> MSSSFVSNGASLEDCHCNLFCLADLTGIKWKRYVWQGPTSAPILFPVTEEDPILSSFSRCLKADVLGVWRRDQRPGRRELWIFWWGKDPNFADLIHHDLSEEEDGVWENGLSYECRTLLFKAVHNLLERCLMNRNFVRIGKWFVKPYEKDEKPINKSEHLSCSFTFFLHGDSNVCTSVEINQHQPVYLLSEEHVTLAQQSNSPFQVILSPFGLNGTLTGQAFKMSDSATKKLIGEWKQFYPISCGLKEMSEEKQDDMDWEDDSLAAVEVLVAGVRMIYPACFVLVPQSDIPAPSSVGASHCSASCLGIHQVPASTRDPAMSSVTLTPPTSPEEVQTVDPQSAQKWVKFSSVSDGFSTDSTSHHGGKIPRKLANHVVDRVWQECNMNRLQNKRKYSATSSGLCEEETADKIGCWDFVEATQRTSCSCLRHKSLKTRNTGQQGQAPSLGQQQQVLPKHKTNEKQDKSEKPQKRPLTPFHHRVSVSDEIGMDTDSASQRLVISAADSQVRFSNIRTNDVAKTPQMHGTELANSPQPPPLSPHPCDVVDEGVTKTPSTPQSQHFYQMPTPDPLVPTKPMEDRIDSLSQSFPPPFQEAVEPTVYVGTAVSLEEDEANVAWKYYKVPKKKDVEFLPPQLPNDKFKDDPVGPFGQESVTSVTELMVQCKKPLKVSDEIVQQYQIKNQYLSAIASDTEQEPKIDPYAFVEGDEEFIFTDKKDRQNSEREAGKKHKVEDGTSAVTVLSHEEDAMSLFSPSKQDAPRPTNHARPPSTSLIYDSDLAVSYTDLDNLFNSDEDELTPGSKKSASGSDDKASSKESKTGNLDPLSCISTADLHKMYPTPPSLEQHIMGFSPMNMNNKEYGSVDTAPGGTVLEGNSSSVGTQFRIEVEEGFCSPKPSEIKDFSYVYKPENCQVLVGCSMFAPLKTLPSHCLPPIKLPEECVYRQSWTVGKLDLLPSGPSMPFIKEGDGSNLDQDYGPAYTPQTHASFGMPPSSAPPSNGGAGILPSPSTPRFPTPRTPRTPRTPRGAGGPASAQGSVKYENSDLYSPASTPSTCRPLNSVEPATVPSIPEAHSLYVNLILSESVMNLFKDCNFDSCCICVCNMNIKGADVGVYIPDPTQEAQYRCTCGFSAVMNRKFGNNSGLFLEDELDIIGRNTDCGKEAEKRFEALRASSVENVNGGLKESEKVPDELILLLQDQCTNLFSPFGAADQDPFPKVGISSNWVRVEERDCCSDCCLALEHGRQFMDNMSGGKVDEALVRSSCLHPWAKQNDASVQCSQDILRMLLSLQPVLQDAIQKKRTVRPWGVQGPLTWQQFHKMAGRGSYGTDESPEPLPIPTFLLGYDYDFLVLSPFALPYWEKLMLEPYGSQRDIAYVVLCPENEALLNGARSFFRDLTAIYESCRLGQHRPISRLLTDGIMKVGATASKKLSEKFVTEWFSQAADGNNEAFSKLKLYAQVCRYDLGPYLASQPLDSSLLSQPNLVAPPNQSLVTAPQMTNTGNANAPSATLASAASSTMTMTSGVPISTSVATANSTLTTTSSSSSSSLSSGVSSNKLPSFPPFGSMNTSGTGSMSAQASTVQSGQLGGQQSSSLQAAGISGESASLPTQPHPDVSESTMDRDKVGIPTDGDSHAITYPPAIVVYIIDPFTYENKDESTNSSNVWTLGLLRCFLEMVQTLPPHIKSTVSVQIVPCQYLLQPVKHDDRQIYSQHLKSLAFSVFTQCRRPLPTSTNVKTLTGFGPGLAMETALKSPDRPECIRLYTPPFILAPVKDKQTELGETFGEAGQKYNVLFVGYCLSHDQRWILASCTDLYGELLETCIINIDVPNRARRKKGSARRFGLQKLWEWCLGLVQMSSLPWRVVIGRLGRIGHGELKDWSCLLSRRNLQSLSKRLKDMCRMCGISAADSPSILSACLVAMEPQGSFVIMPDSVSTGSVFGRSTTLNMQTPQLNTPQDTSCTHILVFPTSASVQVASATYTTENLDLAFNPNNDGADGMGIFDLLDTGDDLDPDIINILPASPTASPVHSPGSHYPHGGDAGKGQGTDRLLSTESHDEVTNILQQPLALGYFVSTAKAGPLPDWFWSACPQAQYQCPLFLKASLHLHVPSVQSDELLHSKHSHPLDSNQTSDVLRFVLEQYNALSWLTCDPAVQDRRSCLPVHFVVLNQLYNFIMNML;> MKAQGETEDSERLSKMSSLLERLHAKFNQNRPWSETIKLVRQVMEKRVVMSSGGHQHLVSCLETLQKALKVTSLPAMTDRLESIARQNGLGSHLSASGTECYITSDMFYVEVQLDPAGQLCDVKVAHHGENPVSCPELVQQLREKNFEEFSKHLKGLVNLYNLPGDNKLKTKMYLALQSLEQDLSKMAIMYWKATNAAPLDKILHGSVGYLTPRSGGHLMNMKYYASPSDLLDDKTASPIILHEKNVPRSLGMNASVTIEGTSAMYKLPIAPLIMGSHPADNKWTPSFSAVTSANSVDLPACFFLKFPQPIPVSKAFVQKLQNCTGIPLFETPPTYLPLYELITQFELSKDPDPLPLNHNMRFYAALPGQQHCYFLNKDAPLPDGQSLQGTLVSKITFQHPGRVPLILNMIRHQVAYNTLIGSCVKRTILKEDSPGLLQFEVCPLSESRFSVSFQHPVNDSLVCVVMDVQDSTHVSCKLYKGLSDALICTDDFIAKVVQRCMSIPVTMRAIRRKAETIQADTPALSLIAETVEDMVKKNLPPASSPGYGMTTGNNPMSGTTTPTNTFPGGPITTLFNMSMSIKDRHESVGHGEDFSKVSQNPILTSLLQITGNGGSTIGSSPTPPHHTPPPVSSMAGNTKNHPMLMNLLKDNPAQDFSTLYGSSPLERQNSSSGSPRMEMCSGSNKAKKKKSSRVPPDKPKHQTEDDFQRELFSMDVDSQNPMFDVSMTADALDTPHITPAPSQCSTPPATYPQPVSHPQPSIQRMVRLSSSDSIGPDVTDILSDIAEEASKLPSTSDDCPPIGTPVRDSSSSGHSQSALFDSDVFQTNNNENPYTDPADLIADAAGSPNSDSPTNHFFPDGVDFNPDLLNSQSQSGFGEEYFDESSQSGDNDDFKGFASQALNTLGMPMLGGDNGEPKFKGSSQADTVDFSIISVAGKALGAADLMEHHSGSQSPLLTTGELGKEKTQKRVKEGNGTGASSGSGPGSDSKPGKRSRTPSNDGKSKDKPPKRKKADTEGKSPSHSSSNRPFTPPTSTGGSKSPGSSGRSQTPPGVATPPIPKITIQIPKGTVMVGKPSSHSQYTSSGSVSSSGSKSHHSHSSSSSSLASASTSGKVKSSKSEGSSSSKLSGSMYASQGSSGSSQSKNSSQTGGKPGSSPITKHGLSSGSSSTKMKPQGKPSSLMNPSISKPNISPSHSRPPGGSDKLASPMKPVPGTPPSSKAKSPISSGSSGSHVSGTSSSSGMKSSSGSASSGSVSQKTPPASNSCTPSSSSFSSSGSSMSSSQNQHGSSKGKSPSRNKKPSLTAVIDKLKHGVVTSGPGGEDPIDSQMGASTNSSNHPMSSKHNTSGGEFQSKREKSDKDKSKVSASGGSVDSSKKTSESKNVGSTGVAKIIISKHDGGSPSIKAKVTLQKPGESGGDGLRPQIASSKNYGSPLISGSTPKHERGSPSHSKSPAYTPQNVDSESESGSSIAERSYQNSPSSEDGIRPLPEYSTEKHKKHKKEKKKVRDKDRDKKKSHSMKPENWSKSPISSDPTASVTNNPILSADRPSRLSPDFMIGEEDDDLMDVALIGN;> MAASSSGEKEKERMGGVSGMAGLGSTRERLLSALEDLEVLSRELIEMLAISRNQKLLQLEEENQVLELLIHRDGDFQELMKLALNQGKVHHEMQALEKEVEKRDSDIQQLQKQLKEAEQILATAVYQAKEKLKSIEKARKGAISSEEIIKYAHRISASNAVCAPLTWVPGDPRRPYPTDLEMRSGLLGQMNNPSTSGVNGHLPGDALAAGRLPDVLAPQYPWQSNDMSVNMLPPNHSSDFLLEPPGHNKENEDDVEVMSTDSSSSSSDSD;> MAAVDIRDNLLGISWVDSSWIPILNSGSVLDYFSERSNPFYDRTCNNEVVKMQRLTLEHLNQMVGIEYILLHAQEPILFIIRKQQRQSPAQVIPLADYYIIAGVIYQAPDLGSVINSRVLTAVHGIQSAFDEAMSYCRYHPSKGYWWHFKDHEEQEKVKPKAKRKEEPSSIFQRQRVDALLIDLRQKFPPRFVQQKSGEKPVPVDQAKKEAEPLPETVKSEEKESTKNIQQTVSTKGPPEKRMRLQ;> MGEPQQVSALPPPPMQYIKEYTDENIQEGLAPKPPPPIKDSYMMFGNQFQCDDLIIRPLESQGIERLHPMQFDHKKELRKLNMSILINFLDLLDILIRSPGSIKREEKLEDLKLLFVHVHHLINEYRPHQARETLRVMMEVQKRQRLETAERFQKHLERVIEMIQNCLASLPDDLPHSEAGMRVKAEPMDTDDNSNCPGQNEQQRESSGHRRDQIIEKDAALCVLIDEMNERP;> MQREEKQLEASLDALLNQVADLKNSLGSFIYKLENEYDRLTWPSVLDSFALLSGQLNTLNKVLKHEKTPLFRNQVIIPLVLSPDRDEDLMRQTEGRVPVFSHEVVPDHLRTKPDPEVEEQEKQLTTDAARIGADAAQKQIQSLNKMCSNLLEKISKEERESESGGLRPNKQTFNPGDTNALVAAVAFGKGLSNWRPSGSSGPGQPGQPGAGTILAGASGLPQVQMPGAPNQQQPMLSGVQMAQAGQPGKMPSGIKTNIKSASMHPYQR;> MASSGVAGGRQAEDTLQPPPELLPESKPPPPPQPLPVAALPPPAAPRPQSPAGAKEENYSFLPLVHNVIKCMDKDSPDLHQDLNALKTKFQELRKLIGTMPGIHVSPEQQQQQLHSLREQVRTKNELLQKYKSLCMFEIPKD;> MAEKFDHLEEHLEKFVENIRQLGIIVSDFQPSSQAGLSQKLNFIVTGLQDIDKCRQQLHDITVPLEVFEYIDQGRNPQLYTKECLERALAKNEQVKGKIDTMKKFKSLLIQELSKVFPEDMAKYRSIRGEDHPPS;> MATYSLANERLRALEDIEREIGAILQNAGTAILELSKEKTNERLLDRQAAAFTTSVQHVEAELSAQIRYLTQVATGQPHEGSSYSSRKDCQMALKRVDYARLKISDVARTCEQMLEN;> MAPVQLDNHQLIPPGGGGGSSGGGGSSSGSASAPAPPPPAAAVAAAAAAAASPGYRLSTLIEFLLHRAYSELMVLTDLLPRKSDVERKIEIVQFASRTRQLFVRLLALVKWANDAGKVEKCAMISSFLDQQAILFVDTADRLASLARDALVHARLPSFAIPYAIDVLTTGSYPRLPTCIRDKIIPPDPITKIEKQATLHQLNQILRHRLVTTDLPPQLANLTVANGRVKFRVEGEFEATLTVMGDDPEVPWRLLKLEILVEDKETGDGRALVHSMQIDFIHQLVQSRLFADEKPLQDMYNCLHCFCLSLQLEVLHSQTLMLIRERWGDLVQVERYHAGKSLSLSVWNQQVLGRKTGTASVHKVTIKIDENDVSKPLQIFHDPPLPASDSKLVERAMKIDHLSIEKLLIDSVHARAHQRLQELKAILRSFNANESSSIETALPALIVPILEPCGNSECLHIFVDLHSGMFQLMLYGLDPATLEDMEKSLNDDMKRIIPWIQQLKFWLGQQRCKQSIKHLPTITTETLQLANYSTHPIGSLSKNKLFIKLTRLPQYYIVVEMLEVPNKPTQLSYNYYFMSVSTADREDSPVMALLLQQFKDNIQDLMSYTKTGKQTRTGTKHKLSDDPCPIDSKKAKRSGEMCAFNKVLAHFVAMCDTNMPFVGLRLELSNLEIPHQGVQVEGDGFNHAIRLLKIPPCKGISEETQKALDRSLLDCTFRLQGRNNRTWVAELVFANCPLNGTSTREQGPSRHVYLTYENLLSEPVGGRKVVEMFLNDWSSIARLYECVLEFARSLPEIPAHLNIFSEVRVYNYRKLILCYGTTKGSSISIQWNSIHQKFHIALGTVGPNSGCSNCHNTILHQLQEMFNKTPNVVQLLQVLFDTQAPLNAINKLPTVPMLGLTQRTNTAYQCFSILPQSSTHIRLAFRNMYCIDIYCRSRGVVAIRDGAYSLFDNSKLVEGFYPAPGLKTFLNMFVDSNQDARRRSVNEDDNPPSPIGGDMMDSLISQLQPPQQQPFPKQPGTSGAYPLTSPPTSYHSTVNQSPSMMHTQSPGNLHAASSPSGALRAPSPASFVPTPPPSSHGISIGPGASFASPHGTLDPSSPYTMVSPSGRAGNWPGSPQVSGPSPATRLPGMSPANPSLHSPVPDVSHSPRAGTSSQTMPTNMPPPRKLPQRSWAASIPTILTHSALNILLLPSPTPGLVPGLAGSYLCSPLERFLGSVIMRRHLQRIIQQETLQLINSNEPGVIMFKTDALKCRVALSPKTNQTLQLKVTPENAGQWKPDELQVLEKFFETRVAGPPFKANTLIAFTKLLGAPTHILRDCVHIMKLELFPDQATQLKWNVQFCLTIPPSAPPIAPPGTPAVVLKSKMLFFLQLTQKTSVPPQEPVSIIVPIIYDMASGTTQQADIPRQQNSSVAAPMMVSNILKRFAEMNPPRQGECTIFAAVRDLMANLTLPPGGRP;> MDVSGQETDWRSAAFRQKLVSQIEDAMRKAGVAHSKSSKDMESHVFLKAKTRDEYLSLVARLIIHFRDIHNKKSQASVSDPMNALQSLTGGPTPGAAGIGMPPRGPGQSLGGMGGLGAMGQPLPLSGQPPPGTSGMAPHGMAVVSTATPQTQLQLQQVALQQQQQQQQQQQFQQQQAALQQQQQQQQQQQQQQQFQAQQNAMQQQFQAVVQQQQLQQQQQQQHLIKLHHQSQQQQIQQQQLQRMAQLQLQQQQQQQQQQALQAQPPMQQPSMQQPQPPPSQALPQQLSQLHHPQHHQPPPQAQQSPIAQNQPPQIPPQSQSQPLVSQAQALPGPMLYAAQQQLKFVRAPMVVQQPQVQPQVQQVQPQVQPQAAVQAAQSAQMVAPGVQMIAEALAQGGMHVRARFPPTSTMSAGPSSSISLGGQPTTQVSQSSLTMLSSPSPGQQVQTPQSMPPPPQPSPQPGSQPNSNVSSGPAPSPSSFLPSPSPQPSQSPVTARTPQNFSVPSPGPLNTPVNPSSVMSPAGSSQAEEQQYLDKLKQLSKYIEPLRRMINKIDKNEDRKKDLSKMKSLLDILTDPSKRCPLKTLQKCEIALEKLKNDMAVPTPPPPPVLPTKQQDLCQPLLDAVLANIRSPVFNHSLYRTFVPAMMAIHGPPIVSPVVCSRKRRFEEDERQSIPNVLQGEVARLDPKFLVNLDPSHCSNNGTVHLICKLDDKDLPSVPPLELSVPADYPAQSPMWIDRQWQYDANPFLQSVHRCMTSRLLQLPDKHSVTALLNTWAQSIHQACLSAA;> MDLAYVCEWEKWAKSTYCPSLPLACAWSCRNLIAFTTDLRNDDQDLTHMIHILDTEHPWEVHSVSSGHSEAITCLEWDQSGSRLLSADADGQIKCWSMADHLANSWESSVGSQVEGDPIVALSWLHNGVKLALHVEKSGASSFGEKFSRVKFSPSLTLFGGKPMEGWIAVTVSGLVTVSLLKPSGQVLTSTESLCRLRGRVALADIAFTGGGNIVVAAADGSSASPVKFYKVCVSVVSEKCRIDTEILPSLFMRCTTDPNRKDRFPAITHLKFLARDMSEQVLLCASSQTSSLVECWSLRKEGLPVNNIFQQISPVVGDKQPMILKWRILSATNDLDRVSAVALPKLPISLTNTDLKVASDTQFYPGLGLALAFQDGSVHMVHRLSLQTMAVFYSSAPRSLDEPALKRPRTTCPAVHFKAMQLSWTSLALVGIDNHGKLSMLRISPSLGHPLEPKLALQHLLFLLEYCMVTGYDWWDILLHVQPGMVQSLVERLHEEYTRQKPALQQVLSTRILAMKASLCKLSPCTVARVCDYHTKLFLMAITSTLKSLLRPHFLNTPDKSPGDRLAEICAKITDVDIDKVMINLKTEEFVLDMNTLQALQQLLQWVGDFVLYLLVSLPNQGSPLRPGHSFLRDGTSLGMLRELMVVIRIWGLLKPSCLPVYTATSDTQDSMSLLFRLLTKLWICCRDEGAASEPDEGLVDECCLLPSQLLVPNLDWLPASDGLVSRLQPKQPLRLRFGRAPTLPSSTSTLQLDGLTRAPGQPKIDHLRRLHLGAYPTEECKACTRCGCVTMLKSPNKTTAVTQWEQRWIKNCLCGGLWRRVPLSCS;> MSGVRAVRISIESACEKQVQEVGLDGTETYLQPLSMSQNLARLAQRIDFSQGSGSEEEEAAGPDGDAPDWGGAGADQDDEEGLVKFQPSLWPWDSVRNNLRSALTEMCVLYDVLSIVRDKKFMTLDPVSQDALPPKQSPQTLQLISKKKSLAGAAQILLKGAERLTKSVAENQENKLQRDFNSELLRLRQHWKLRKVGDKILGDLSYRSAGSLFPHHGTFEVIKNTDIDLDKKIPEDYCPLDVQIPSDLEGSAYIKVSIQKQAPDIGDLGTVNLFKRPLPKSKPGSPHWQTKLEAAQNVLLCKEIFAQLSREAVQIKSQIPHIVVKNQIISQPFPSLQLSISLCHSSDDKKSQKCAAEKPGQEDHLYVLEHNLHLLIREFHKQTLSSIVMPHPASAPFGHKRMRLSGPQAFDKNEINSIQSTEGLLEKIIKQAKHIFLRSRTAATIDSLASRIEDPQIQAHWSNINDVYESSVKVLITSQGYEQICKSIQLQLNIGVEQVRVVHRDGRVIMLSHQEQELQDFLLSQMSQHQVHAVQQLAKVMGWQVLSFSNHVGLGPIESIGNASAITVASPSGDYAISVRNGPESGSKIMVQFPRNQCKDLPKSDVLQDSKWSHLRGPFKEVQWNKMEGRNFVYKMELLMSALSPCLL;> MEAPPVTMMPVTGGTINMMEYLLQGSVLDHSLESLIHRLRGLCDNMEPETFLDHEMVFLLKGQQASPFVLRARRSMDRAGAPWHLRYLGQPEMGDKNRHALVRNCVDIATSENLTDFLMEMGFRMDHEFVAKGHLFRKGIMKVVVYKIFRILVPGNTDSTEALSLSYLVELSVVAPAGQDMVSDDMRNFAEQLKPLVHLEKIDPKRLM;> MGVTCVSQMPVAEGKSLQQTVELLTKKLEMLGAEKQGTFCVDCETYHTAASTLGSQGQAGKLMYVMHNSEYPLSCFALFENGPCLIADTNFDVLMVKLKGFFQSAKASKIETRGTRYQYCDFLVKVGTVTMGPSARGISVEVEYGPCVVASDCWSLLLEFLQSFLGSHAPGAPTVFGNRHDAVYGPADTMIQYMELFNKIRKQQQVPVAGIR;> MADRLTQLQDAVNSLADQFCNAIGVLQQCGPPASFSNIQTAINKDQPANPTEEYAQLFAALIARTAKDIDVLIDSLPSEESTAALQAASLYKLEEENHEAATCLEDVVYRGDMLLEKIQSALADIAQSQLKTRSVTHSHSLPDS;> MAQQRALPQSKETLLQSYNKRLKDDIKSIMDNFTEIIKTAKIEDETQVSRATQGEQDNYEMHVRAANIVRAGESLMKLVSDLKQFLILNDFPSVNEAIDQRNQQLRALQEECDRKLITLRDEVSIDLYELEEEYYSSSSSLCEANDLPLCEAYWRLDLDADSADGLSAPLLASPETGAGPLQSAAPVHSHGGGPGPTEHT;> METQLQSIFEEVVKTEIIEEAFPGMFMDTPEDEKTKLISCLAAFRQFWSGLSQESHEQCVQWIVKFIHGQHSPKRISFLYDCLAMAVETGLLPPRMVCESLINSDSLEWERTQLWALTFKLVRKIIGGVDYKGVRDLLKAILEKILTIPNTVSSAVVQQLLAAREVIAYILERNACLLPAYFAVTEIRKLYPEGKLPHWLLGNLVSDFVDTFRPTARINSICGRCSLLPVVNNSGAICNSWKLDPATLRFPLKGLLPYDKDLFEPQTALLRYVLEQPYSRDMVCNMLGLNKQHKQRCPVLEDQLVDLVVYAMERSETEEKFDDGGTSQLLWQHLSSQLIFFVLFQFASFPHMVLSLHQKLAGRGLIKGRDHLMWVLLQFISGSIQKNALADFLPVMKLFDLLYPEKECIPVPDINKPQSTHAFAMTCIWIHLNRKAQNGDSTLQIPIPHSLKLHHEFLQQSLRNKSLQMNDYKIALLCNAYSTNSECFTLPMGALVETIYGNGIMRVPLPGTSCLASASVTPLPMNLLDSLTVHAKMSLIHSIATRVIKLAHTKSSVALAPALVETYSRLLVYMEIESLGIKGFISQLLPTVFKSHAWGILHTLLEMFSHRMHHIQPHYRVQLLSHLHTLAAVAQTNQNQLHLCVESTALRLITALGSSEVQPQFTRFLNDPKTVLSAESEELNRALILTLARATHVTDFFTGSDSIQGTWCKDILQTIMNFTPHNWASHTLSCFPAPLQAFFKQNNVPQESRFNLKKNVEEEYRKWKSMTDENEIITQFSVQGFPPLFLCLLWKMLLETDHISQIGYKVLERIGARALVAHVRTFADFLVYEFSTSAGGQQLNKCIEILNDMVWKYNIVTLDRLILCLAMRSHEGNEAQVCYFIIQLLLLKPNDFRNRVSDFVKENSPEHWLQSDWHTKHMSYHKKYPEKLYFEGLAEQVDPPVPIQSPYLPIYFGNVCLRFLPVFDIVIHRFLELLPVSKSLETLLDHLGGLYKFHDRPVTYLYNTLHYYEMCLRNRDHLKRKLVHAIIGSLKDNRPQGWCLSDTYLKHAMNAREDNPWVPEDSYYCKLIGRLVDTMAGKSPGPFPNCDWRFNEFPNPAAHALHVTCVELMALAVPGKDVGNALLNVVLKSQPLVPRENITAWMNAIGLIITALPEPYWIVLHDRIVNVISSSSLTSETEWVGYPFRLFDFTACHQSYSEMSCSYTLALAHAVWHHSSIGQLSLIPKFLTEALLPVVKTEFQLLYVYHLVGPFLQRFQQERTRCMIEIGVAFYDMLLNVDQCSTHLNYMDPICDFLYHMKYMFTGDSVKEQVEKIICNLKPALKLRLRFITHISKMEPAVPPQALNSGSPAPQSNQVPASLPVTQ;> MKVVNLKQAILQAWKERWSDYQWAINMKKFFPKGATWDILNLAEALLEQAMIGPSPNPLILSYLKYAISSQMVSCSSVLTAISKFDDFSRDLCVQALLDIMDMFCDRLSCHGKAEECIGLCRALLSALHWLLRCTAASAERLQEGLEAGTPAPGEKQLALCLQCLEKTLSSTKNRALLHIAKLEEASSWTAIEHSLLKLGEILANLSNPQLRSQAERCGTLIRSIPSMLSVHSEQLHKTGFPTIHALILLEGTMNLTGEMQPLVEQLMMVKRMQHIPTPLFVLEIWKACFVGLIESPEGTQELKWTAFTYLKIPQVLVKLKKYFHGEKDFTEDVNCAFEFLLKLTPLLDKADQRCNCDCTNFLLQECNKQGLLSEVNFASLVGKRTADRDPQLKSSENANIQPNPGLILRAEPTVTNILKTMDADHSKSPEGLLGVLGHMLSGKSLDLLLAAAAATGKLKSFARKFINLNEFTTHGSGESTKTASVRALLFDISFLMLCHVAQTYGSEVILSESSSGEEVPFFETWMQTCMPEEGKILNPDHPCFRPDSTKVESLVALLNNSSEMKLVQMKWHEACLSISAAILEILNAWENGVLAFESIQKITDNIKGKVCSLAVCAVAWLVAHVRMLGLDEREKSLQMIRQLAGPLYSENTLQFYNERVVIMNSILEHMCADVLQQTATQIKFPSTGVDTMPYWNLLPPKRPIKEVLTDIFAKVLEKGWVDSRSIHILDTLLHMGGVYWFCNNLIKELLKETRKEHTLRAVQLLYSIFCLDMQQVTLVLLGHILPGLLTDSSKWHSLMDPPGTALAKLAVWCALSSYSSHKGQASSRQKKRHREDIEDYVSLFPVEDMQPSKLMRLLSSSDDDANILSSPTDRSMNSSLSASQLHTVNMRDPLNRVLANLFLLISSILGSRTAGPHTQFVQWFMEECVGCLEQDSRGSILQFMPFTTVSELVKVSAMSSPKVVLAITDLSLPLGRQVAAKAIAAL;> MVPGSEGPARAGGLVADVVFVIEGTANLGPYFEELRKHYLLPAIEYFNGGPPAETDFGGDYGGTQYSLVVFNTVDCAPESYVQCHAPTSSAYEFVTWLDGIKFMGGGGESCSLIAEGLSTALQLFDDFKKMREQIGQTHRVCLLICNSPPYLLPAVESTTYSGCTTESLVQKIGERGIHFSIVSPRKLPALRLLFEKAAPPALLEPLQQPADVSQDPRHMVLVRGLVLPVGGSSTSGSLQTKQAVPLPPAPASAATLSAAPPQALPPVPPQYQVPGNLSAAQVAAQNAVEAAKSQKAGLGPRFSPINPLQQAAPGVGPPFSQAPAPPLAPVPPGAPKPPPASQPSLVSTVAPGPVLAAPAQPGAPSLAGTVTPGGVNGPSAAQLGGPALGGQQSVSNKLLAWSGVLEWQEKPKPASVDANTKLTRSLPCQVYVNHGENLKTEQWPQKLIMQLIPQQLLTTLGPLFRNSRMVQFHFTNKDLESLKGLYRIMGNGFAGCVHFPHTAPCEVRVLMLLYSSKKKIFMGLIPYDQSGFVNGIRQVITNHKQVQQQKLEQQRGMGAQQAPPVLGPILEEQARPPQNLLQLRAPQPQPQGAVGASAATGQPQPQGATQAPTGAPQGPPGAAPGPPPSGPILRPQNPGANPQLRSLLLNPAPPQTGVPPPQASLHHLQPPGAPTLLPPHQSMGQPQLGPQLLHPPPAQSWPTQLPQRAPLPGQMLLSGGPRGPVPQPGLQPSVMEDDILMDLI;> MADVLSVGVNLEAFSQAISAIQALRSSVSRVFDCLKDGMRNKETLEGREKAFIANFQDNLHSVNRDLNELERLSNLVGKPSENHPLHNSGLLSLDPVQDKTPLYSQLLQAYKWSNKLQYHAGLASGLLNQQSLKRSANQMGVSAKRRPKAQPTTLVLPPQYVDDVISRIDRMFPEMSIHLSRPNGTSAMLLVTLGKVLKVIVVMRSLFIDRTIVKGYNESVYTEDGKLDIWSKSSYQVFQKVTDHATTALLHYQLPQMPDVVVRSFMTWLRSYIKLFQAPCQRCGKFLQDGLPPTWRDFRTLEAFHDTCRQ;> MAASLGGMFTGQPPGPPPPPPGLPGQASLLQAAPGAPRPSNSTLVDELESSFEACFASLVSQDYVNGTDQEEIRTGVDQCIQKFLDIARQTECFFLQKRLQLSVQKPDQVIKEDVSELRSELQRKDALVQKHLTKLRHWQQVLEDINVQHKKPADMPQGSLAFLEQASANIPAPLKQT;> MAAPQPQAAAVSSASGVSGPGSAGGPGPQQQPQPTQLVGSAQSGLLQQQQQDFDPVQRYKMLIPQLKESLQTLMKVAAQNLIQNTNIDNGQKSSDAPLQRFDKCLEEFYALCDQLELCLRLAHECLSQSCDSAKHSPTLVPTATKPDAVQPDSLPYPQYLAVIKAQITCAKDIHTALLDCANKVTGKTTAPSTGPGGSL;> MSTPPLAPTGMASGPFGGPQAQQAAREVNTATLCRIGQETVQDIVYRTMEIFQLLRNMQLPNGVTYHTGTYQDRLTKLQDHLRQLSILFRKLRLVYDKCNENCGGMDPIPVEQLIPYVDEDGSKNDDRAGP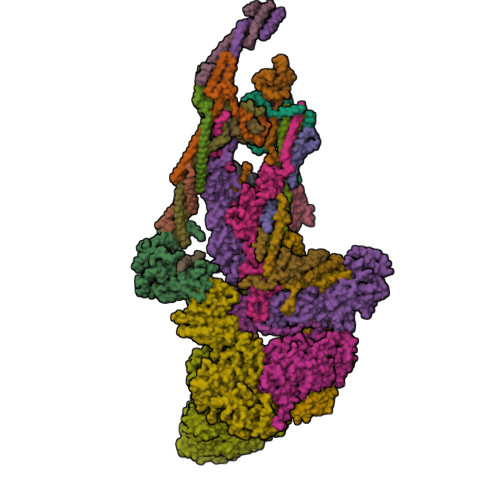PRFASEERREIVEVNKKLKQKNQQLKQIMDQLRNLIWDINAMLAMRN;> MAAAVAMETDDAGNRLRFQLELEFVQCLANPNYLNFLAQRGYFKDKAFVNYLKYLLYWKEPEYAKYLKYPQCLHMLELLQYEHFRKELVNAQCAKFIDEQQILHWQHYSRKRVRLQQALAEQQQQNNTAGK> ENLKDEILEKYIPKTKKTRSGHIVIKTEETPNPEIVANTRTVPGIITARGCAYAGCKGVVMGPIKDMVHITHGPIGCSFYTWGGRRFKSKPENGTGLNFNEYVFSTDMQESDIVFGGVNKLKDAIHEAYEMFHPAAIGVYATCPVGLIGDDILAVAATASKEIGIPVHAFSCEGYKGVSQSAGHHIANNTVMTDIIGKGNKEQKKYSINVLGEYNIGGDAWEMDRVLEKIGYHVNATLTGDATYEKVQNADKADLNLVQCHRSINYIAEMMETKYGIPWIKCNFIGVDGIVETLRDMAKCFDDPELTKRTEE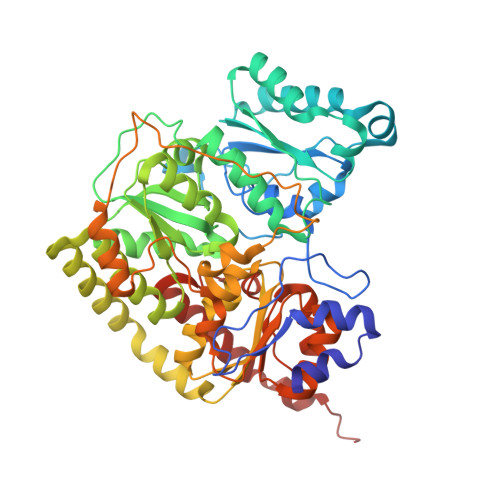VIAEEIAAIQDDLDYFKEKLQGKTACLYVGGSRSHTYMNMLKSFGVDSLVAGFEFAHRDDYEGREVIPTIKIDADSKNIPEITVTPDEQKYRVVIPEDKVEELKKAGVPLSSYGGMMKEMHDGTILIDDMNHHDMEVVLEKLKPDMFFAGIKEKFVIQKGGVLSKQLHSYDYNGPYAGFRGVVNFGHELVNGIYTPAWKMITPPWK4-fluoro-N-{1-[(Z)-iminomethyl]cyclopropyl}-N~2~-{(1S)-2,2,2-trifluoro-1-[4'-(methylsulfonyl)[1,1'-biphenyl]-4-yl]ethyl}-L-leucinamide | 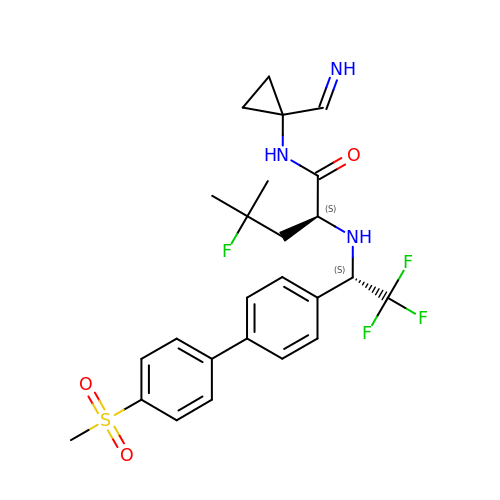C25 H29 F4 N3 O3 S | ZVRLJSQZXQQABF-OLOBTLGRSA-N>MGKGHHHHHHGSERTGTQPLGVQGLTEEQRMMIRELMDAQMKTFDTTFSHFKNFRLPGVLSSGCELPESLQAPSREEAAKWSQVRKDLCSLKVSLQLRGEDGSVWNYKPPADSGGKEIFSLLPHMADMSTYMFKGIISFAKVISYFRDLPIEDQISLLKGAAFELCQLRFNTVFNAETGTWECGRLSYCLEDTAGGFQQLLLEPMLKFHYMLKKLQLHEEEYVLMQAISLFSPDRPGVLQHRVVDQLQEQFAITLKSYIECNRPQPAHRFLFLKIMAMLTELRSINAQHTQRLLRIQDIHPFATPLMQELFGITGS[2x];>CPSSHSSLTERHKILHRLLQEGSPS[2x]

The xenobiotic receptor pregnane X receptor (PXR) is an orphan member of the nuclear receptor superfamily. The activity of human PXR (hPXR) can be induced by many structurally diverse chemicals, leading to the transcriptional upregulation of drug-metabolizing enzymes (e.g., cytochrome P450 3A4 [CYP3A4]) and transporters (e.g., multidrug resistance protein 1 [MDR1]) to enhance the metabolism and excretion of xenobiotics, such as therapeutic agents, and endobiotics, such as steroid hormones, bile acids and glucose. PXR forms heterodimers with retinoid X receptor (RXR) to bind to the promoters of its target genes. The transcriptional activity of PXR is enhanced by co-activators, such as steroid receptor coactivator 1 (SRC-1) and transcriptional mediator/intermediary factor 2 (TIF2), and repressed by co-repressors, such as nuclear receptor corepressor (NCoR) and silencing mediator for retinoid or thyroid hormone receptors (SMRT).

Similarly, we determined the crystal structure of the hPXR LBD in complex with the agonist SJB7 and the co-activator peptide SRC-1 (CPSSHSSLTERHKILHRLLQEGSPS) at a resolution of 2.66 Å. The hPXR LBD displays the canonical α-helical sandwich common to nuclear receptors, along with the characteristic five-stranded antiparallel β-sheet unique to hPXR. The complex exhibits a homodimer in the asymmetric unit, as observed in a number of previously reported hPXR LBD structures, with the dimer interface being formed by the β1′-strands from each monomer. Protein chains A and B are similar in structure, sharing a root mean square deviation of 0.727 Å over all atoms. The hPXR LBD adopts an active conformation with the AF-2 helix (helix 12) positioned to favor co-activator binding, in which the SRC-1 peptide is seen packed against the AF-2 groove of each LBD. SJB7 resides in the highly hydrophobic ligand-binding site, with no hydrogen bond having been clearly observed. The t-butyl group makes hydrophobic contacts with W299, which interacts with most, if not all, of the ligands co-crystallized to date. The ring of the t-butylphenyl group interacts with M243 and M323, with L209, V211, Y306 and L308 providing additional contacts to enclose the t-butylphenyl moiety. The triazole group is fastened in place by a narrow channel that is ~8–9 Å wide and is formed by S247, Q285, H407 and L411, which reflects the plasticity of the hPXR LBD in molding to the shape of the ligand and may contribute to the favorable positioning of key protein–ligand interactions. The dimethoxy-methylphenyl moiety forms π-π interactions with F429, in addition to F281, whereas L428 and F429 form contacts with the para-methoxy group, which is also engaged with A280.> U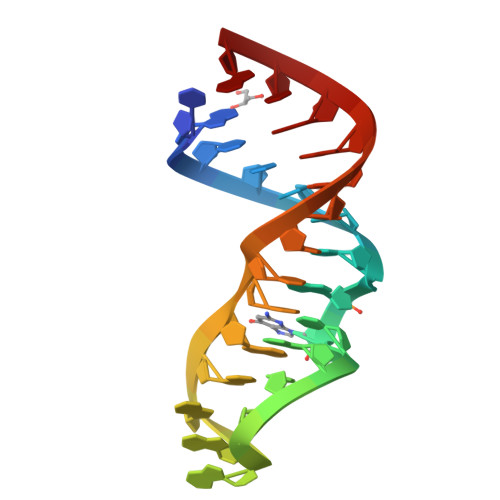GCUCCUAGUACGAGAGGACCGGAGUG(2S)-1-{[(R)-hydroxy{[(1R,2R,3S,4S,5S,6S)-2,3,4,5,6-pentahydroxycyclohexyl]oxy}phosphoryl]oxy}-3-(pentanoyloxy)propan-2-yl decanoate | C24 H45 O13 P | 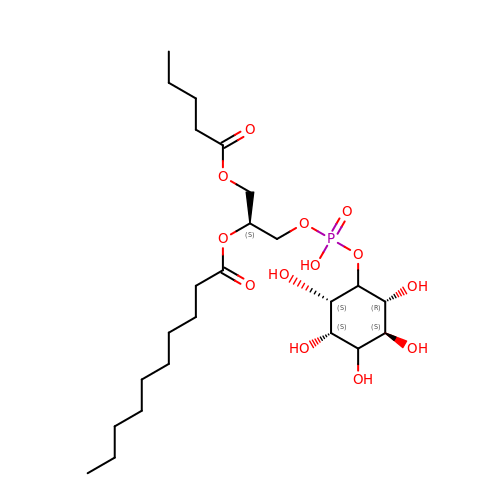YWVFSDQOBMMIAJ-CLASQLQRSA-N>[2x]GMPQPTVLLLARADLSPVGTEFTTGPIDAHDPFDSGRRTAFVDEQGIAAGIVEFGTALSVEAYPYTEMLVMHRGSVTLTSGTD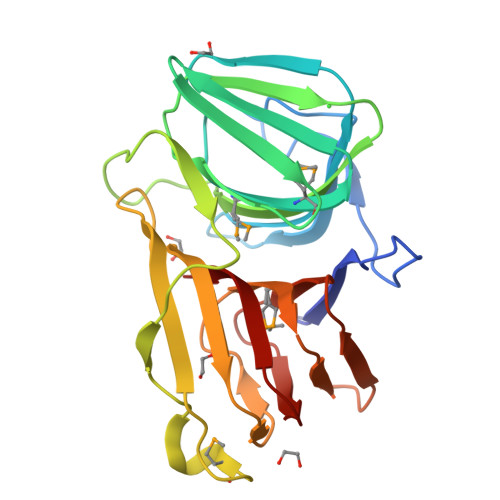SVTLSTGESAVIGRGTQVRIDAQPESLWAFCASTQASGPDKSGITALDRLALLTPSSPPDPSIMISPLPQCRSNNLFEDTASTLRIGVWDSTPYERISRPHKIHELMNLIEGRVVLSLENGSSLTVNTGDTVFVAQGAPCKWTSTGYVRKFYAVT>MGDTAVNVGSAAGTGANTTNTTTQAPQNKPYFTYNNEIIGEATQSNPLGNVVRTTISFKSDDKVSDLISTISKAVQFHKNNSASGENVTINENDFINQLKANGVTVKTVQPSNKNEKAYEAIDKVPSTSFNITLSATGDN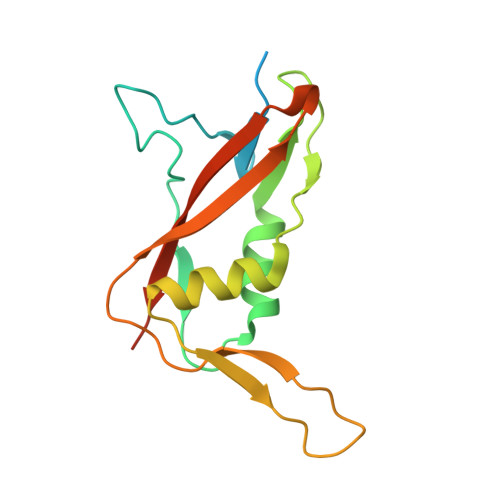NQTATIQIPMVPQGLEHHHHHH[2x]>MNIQKSENKANPQKLVVALLPDESAATVIQNNKGLEMYLENKLNKDIELFVSTDYSSMIEVASKGRLDLAYFGPLSYVLAKTKSNIEPFAALEKDGKNTYQALVIGNAEAGINSYEKIEGKIMAYGDQASTSSHLIPKSMLKQKQLKAGENYEEVFVGAHDAVAIAVANGKAQAGGLSKPIFTALIERGTIDKNKVIIIAESKPFPQYPWTMRSDLDSELKTQIQQAFLELEDKAILKPFKADAFTLVTDQDYDVVRNLGEVLELNFEQLNKLEHHHHHH[2x]

Here we elucidate the molecular basis of high-affinity phosphite and hypophosphite acquisition by determining the ligand-binding affinity and structure of the PBPs of phosphite and hypophosphite ABC transporters from environmental microorganisms. We over-produced and purified PBPs of three putative phosphite transporters; PtxB from the globally important marine diazotroph Trichodesmium erythraeum IMS101 (Te_PtxB), PhnD from the oceanic picocyanobacteria Prochlorococcus marinus MIT9301 (Pm_PhnD)35 and PtxB from the soil bacterium Pseudomonas stutzeri WM88 (Ps_PtxB), as well as a PBP from a putative hypophosphite transporter, HtxB, also from P. stutzeri WM88 (HtxB)18. The structures reveal that ligand specificity, measured here by thermophoresis, arises from a combination of steric considerations and the interaction between a ligand P-H hydrogen atom and an aromatic π system in the binding pocket. The structures of two distinct types of phosphite-binding protein and a hypophosphite-binding protein reveal that a P-H…π interaction ensures high-affinity binding of specific ligands, representing a universal mechanism in these PBPs for recognising ligands with a P-H bond.

To determine the structural mechanism of phosphite selectivity we co-crystallised Te_PtxB and Pm_PhnD with phosphite resulting in high-resolution structures (1.95 and 1.46 Å respectively) of the closed, ligand-bound complexes. In the closed form, the amino acids that form the walls of the binding pocket pack tightly against the phosphite moiety and a single water molecule that is also buried in the binding pocket. Each oxygen atom of the phosphite contributes to an extensive hydrogen bonding network to the main chain and side chains of a cluster of conserved residues from lobe 2 (Te_PtxB; Y55, Y100, S130, T131, S132 and H160; Pm_PhnD; Y46, S126, T127, S128, H158 and D205, Figs. 1d, e and 2e, f). In Te_PtxB, it is not possible to determine the protonation state of the phosphite from the pattern of hydrogen bonding, but given the pH of the crystallisation experiment (pH 4.2), it is also likely that the mono-anionic form of phosphite is bound (phosphite pKa 1.5, 6.739). Both proteins contain a conserved histidine as one of the phosphite ligands (Te_PtxB; H160 and Pm_PhnD; H158), which could help stabilise the negative charge on the phosphite. However, in Te_PtxB, one imidazole nitrogen atom acts as a hydrogen bond acceptor to a mainchain N-H (S178), suggesting that the histidine is neutral. In both structures, the hydrogen atom at the R1 position of the phosphite points towards lobe 1, packing against the face of the aromatic ring of a tyrosine residue (Te_PtxB; Y208, Pm_PhnD; Y206). This tyrosine sidechain forms a cap that is stabilised by intramolecular hydrogen bonds to residues on lobe 1 (Te_PtxB; D22, Pm_PhnD; D13 and N176), which in the closed conformation, contributes to the network of interactions that connect both lobes of the protein and bury the binding pocket from solvent.> MRPEAAAAELRRLLPLLSFAGRRTGAATHSVASLIVSTAYSATAARSVTNHSRDCPVLSKKLPLPLIGKESSFAARPCLNCVRERVHYVSSLSFCDYFEKKCAEAQHYRNGASSNGVVGTAALPKLLLEAIERSYGSVAAFKDSVMLHSTGAMSPGRLWIVYTPPISGSEHGAVRLLNLPACKVPLVHGLWPLAVINMTEKRLCEQIACRSGKGGDAVDADDAPAWRHAARTRKTLGALATTEEGNDRAGNVAQVKLSSIQSAIAEEALCAMNWKFVETQLTSALAYYSSKERTQTQREHRKEKEHVAAVRAMSQLKNSGAVIHATDSVTITSSNSFVASSASEPNLSAAAAVTSSSAKAENSALGEANTQTAAVAAPSAEATAANTASN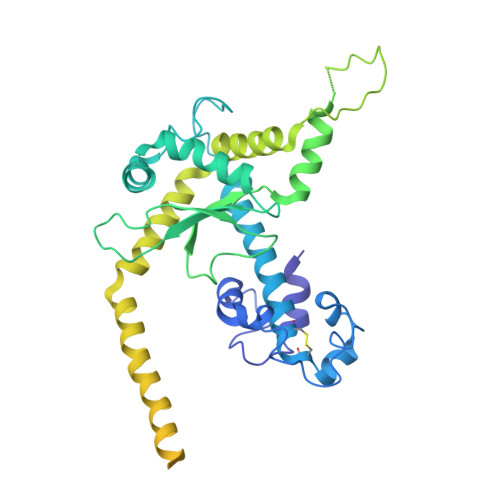SAQPADNTATGAAAAEPRAVQQADGTWEYHYNNGSVTKALPDGTKVFQTESLTTTVFVNGDTLFEYPNNTSILDRADGVRVITYADGTKKEERLK>GSRYQQPPVPYRQIDDCPAKARPQHIFYRRFLGKDGRRDPKCQWKFAVIFWGNDPYGLKKLSQAFQFGGVKAGPVSCLPHPGPDQSPITYCVYVYCQNKDTSKKVQMARLAWEASHPLAGNLQSSIVKFKKPL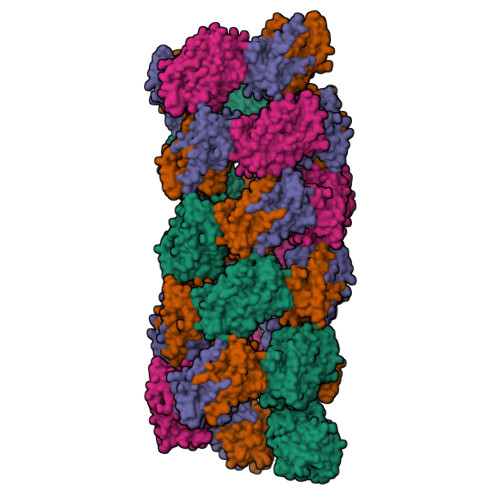PLTQPG[4x]The highly conserved eukaryotic multifunctional polymerase-associated factor 1 (Paf1) complex (Paf1C) was originally identified in budding yeast over 2 decades ago1, and robust data suggested that it plays a vital role in transcriptional elongation and chromatin modifications. In this study, we determine the atomic structures of both the human PAF1/CTR9 and yeast Paf1/Ctr9 heterodimers, both with a resolution of ~2.53 Å. Our analysis revealed that both the hook-shaped (hookfold) PAF1(57–116) and Paf1(34–103) occupied the concave channel and convex surface of the right-handed superhelix-folded CTR9(1–249) and Ctr9(1–313), respectively, with very similar conformations, although the sequence identity was low between human PAF1 and yeast Paf1 or CTR9 and Ctr9. Our results clearly reveal that the heterodimer of PAF1/CTR9 or Paf1/Ctr9 is the core component and is important for human PAF1C or yeast Paf1C assembly, yeast viability, and Paf1C-mediated histone modifications.

Next, we used the same approach by creating a single polypeptide through fusing Ctr9(1–313) to the N-terminus of Paf1(34–103) with a TEV-cleavable segment. The crystal structure of Ctr9(1–313)–Paf1(34–103) was determined at a resolution of 2.53 Å with one molecule in the asymmetric unit. Superimposition of the structures of the yeast Ctr9(1–313)–Paf1(34–103) and human CTR9(1–249)–PAF1(57–116) heterodimers resulted in a root-mean-square deviation of 2.63 Å for 198 equivalent Cα atoms, indicating that human CTR9/PAF1 and yeast Ctr9/Paf1 subcomplexes share similar heterodimer structures. Similar to human CTR9/PAF1 subcomplex interactions, the Ctr9(1–313)/Paf1(34–103) interface could be divided into three regions. In detail, region I was also mainly maintained by hydrophobic interaction through four conserved hydrophobic amino acids in Paf1 and corresponding amino acids in Ctr9, and by hydrogen bonds between D61/Q150 and K191, M64/K191, and D67/N104. Substitution of these four amino acids in Paf1 with serines (L62S, M64S, V66S, and L68S, referred to 4S) led to the complete disruption of Paf1/Ctr9 subcomplex formation (lane 3 in Fig. 4h). In this region, Paf1 had a longer loop than other species (e.g., worm to human), including a shorter α-helix (αC') that bound the N-terminal tail of Ctr9, which is different from human CTR9/PAF1 complex. Notably, the [Ctr9(N16Δ)] mutant did not form complex with Paf1 thoroughly, indicating that this longer N-terminal tail of Ctr9 is essential to maintain the interaction between Ctr9 and Paf1. For region III, D95 was the core amino acid in the C-terminus αD' of Paf1, which bound with R221, R243, and Y10 of Ctr9, mainly mediated by extensive hydrogen bonds. D95K mutation in Paf1 also abolished the interaction between Ctr9 and Paf1 completely (lane 5 in Fig. 4h).

> MTNAMKVEGYPSMEWPTSLDIPLKASEELVGIDLETDLPDDPTDLKTLLVEENSEKEHWLTIALAYCNHGKTNEGIKLIEMALDVFQNSERASLHTFLTWAHLNLAKGQSLSVETKEHELTQAELNLKDAIGFDPTWIGNMLATVELYYQRGHYDKALETSDLFVKSIHAEDHRSGRQSKPNCLFLLLRAKLLYQKKNYMASLKIFQELLVINPVLQPDPRIGIGLCFWQLKDSKMAIKSWQRALQLNPKNTSASILVLLGEFRESFTNSTNDKTFKEAFTKALSDLNNIFSENQHNPVLLTLLQTYYYFKGDENLYFQSETNADSSQLINSLYIKTNVTNLIQQDEDLGMPVDLMKFPGLLNKLDSKLLYGFDNVKLDKDDRILLRDPR>[2x]GSFTMDFPYDLNALFPERISVLDSNLSAGRKAHGRPDPLPQVTTVIDELGKASSKAQQLPAPITSAAKLQANRHHLYLLKDGEQNGGRGVIVGFLKVGYKKLFLLDQRGAHLETEPLCVLAF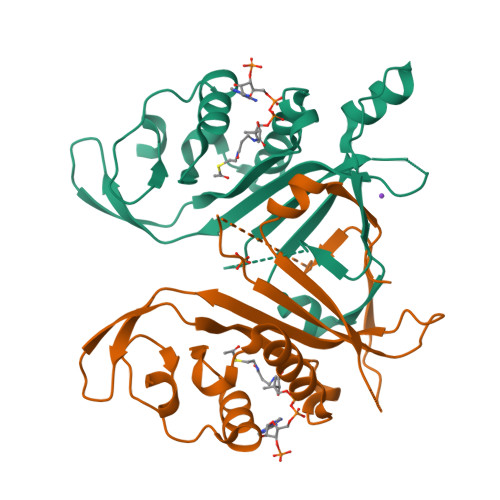YVTETLQRHGYGSELFDFMLKHKQVEPAQMAYDRPSPKFLSFLEKRYDLRNSVPQVNNFVVFAGFFQSRSGTPPSPLT>GPGSDNKEQTTDQPLAKDKVALLIGNMNYREHPKLKAPLVDVYELTNLLRQLDFKVVSLLDLTEYEMRNAVDEFLLLLDKGVYGLLYYAGHGYENFGNSFMVPVDAPNPYRSENCLCVQNILKLMQEKETGLNVFLLDMCRKRNDYDDTIPILDALKVTANIVFGYATCQGAEAFEIQHSGLANGIFMKFLKDRLLEDKKITVLLDEVAEDMGKCHLTKGKQALEIRSSLSEKRALTDPIQGTEYSAESLVRNLQWAKAHELPESMCLKFDCGV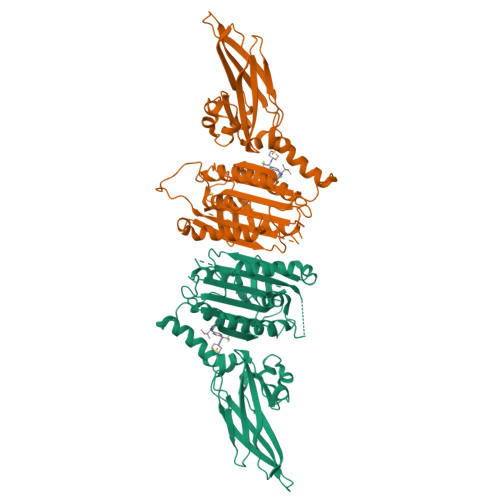QIQLGFAAEFSNVMIIYTSIVYKPPEIIMCDAYVTDFPLDLDIDPKDANKGTPEETGSYLVSKDLPKHCLYTRLSSLQKLKEHLVFTVCLSYQYSGLEDTVEDKQEVNVGKPLIAKLDMHRGLGRKTCFQ[2x]(1R)-2-(1-CARBOXY-2-HYDROXY-2-METHYL-PROPYL)-5,5-DIMETHYL-THIAZOLIDINE-4-CARBOXYLIC 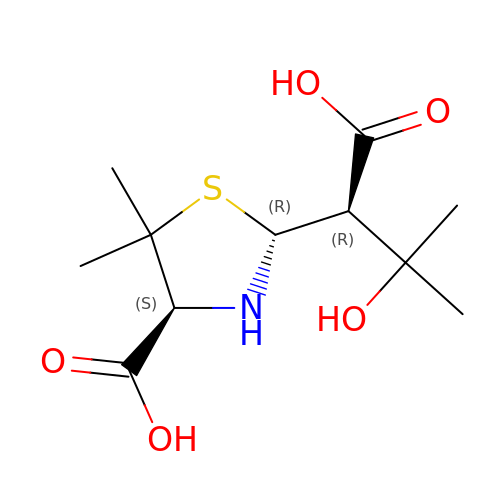ACID | C11 H19 N O5 S | MAATUKZAHQWKEG-LYFYHCNISA-N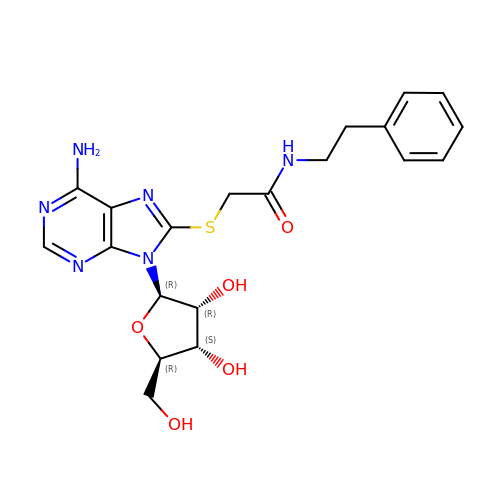8-({2-oxo-2-[(2-phenylethyl)amino]ethyl}sulfanyl)adenosine | C20 H24 N6 O5 S | WAETXEWYOOCYCX-BGIGGGFGSA-N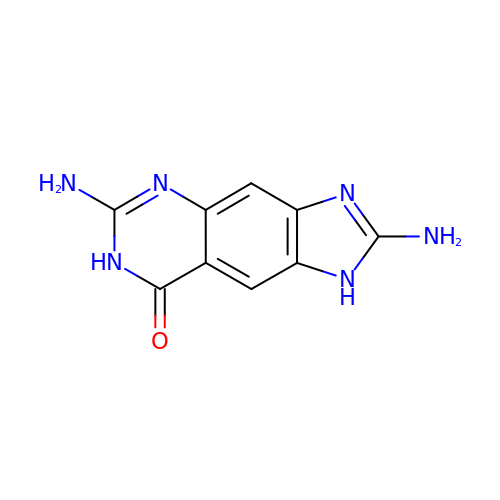2,6-diamino-1,7-dihydro-8H-imidazo[4,5-g]quinazolin-8-one | C9 H8 N6 O | WFECBOHPSURSGU-UHFFFAOYSA-N>AQVINTFDGVADYLQTYHKLPDNYITKSEAQALGWVASKGNLADVAPGKSIGGDIFSNREGKLPG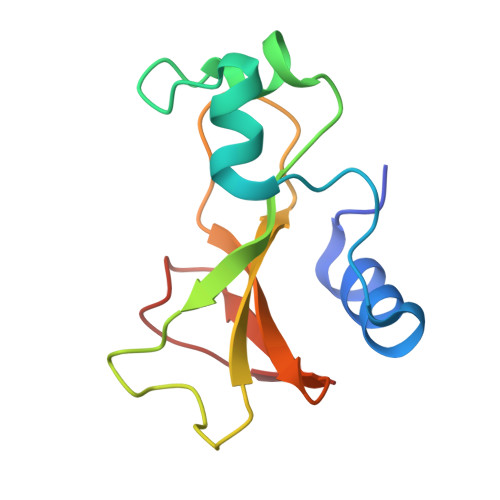KSGRTWREADINYTSGFRNSDRIVYSSDWLIYKTTDHYQTFTKIR[3x]> GPGSMGVPICGACRRPIEGRVVNAMGKQWHVEHFVCAKCEKPFLGHRHYERKGLAYCETHYNQLFGDVCFHCNRVIEGDVVSALNKAWCVNCFACS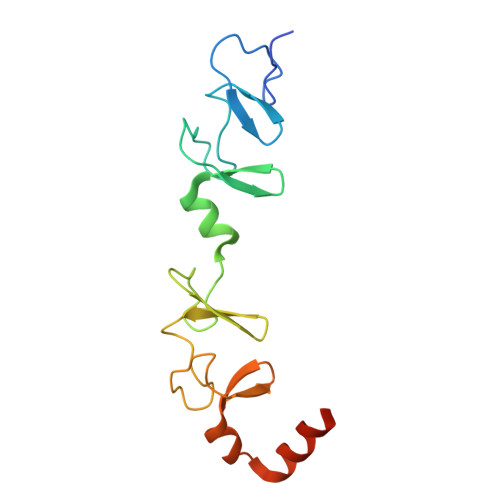TCNTKLTLKNKFVEFDMKPVCKKCYEKFPLELKKRLKKLAETLGRK>[8x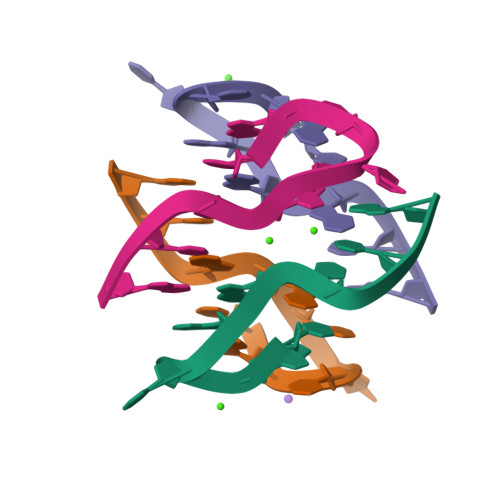]CGTCAGGCG> HVFIRTELSFIKNNVPCIRDMFFIYKRELYNICLDDLKGEEDETHIYVQKKVKDSWITLNDLFKETDLTGRPHIFAYVDVEEIIILLCEDEEFSNRKKDMTCHRFYSNDGKEYQNSEITISDYILKDKLLSSYVSLPLKIENREYFLICGVSPYKFK;> HVFIRTELSFIKNNVPCIRDMFFIYKRELYNICLDDLKGEEDETHIYVQKKVKDSWITLNDLFKETDLTGRPHIFAYVDVEEIIILLCEDDEFSNRKKDMTCHRFYSNDGKEYQNSEITISDYILKDKLLSSYVSLPLKIENREYFLICGVSPYKFKDDNK;> DDNKKDDILCMASHDKGETWGTKIVIKYDNYKLGVQYFFLRPYISKNDLSFHFYVGDNINNVKNVNFIECTHEKDLEFVCSNRDFLKDNKVLQDVSTLNDEYIVSYGNDNNFAECYIFFNNENSILIKPEKYGQTTAGCYGGTFVKIDEQRTLFIYSSSQGIYNIHTIYYANYEEF;> KDDILCMASHDKGETWGTKIVIKYDNYKLGVQYFFLRPYISKNDLSFHFYVGDNINNVKNVNFIECTHEKDLEFVCSNRDFLKDNKVLQDVSTLNDEYIVSYGNDNNFAECYIFFNNENSILIKPEKYGNTTAGCYGGTFVKIDEQRTLFIYSSSQGIYNIHTIYYANYE

Sequencing and annotation of the P. falciparum genome has supported the identification of new blood-stage vaccine candidate antigens, among which the P. falciparum Cysteine-Rich Protective Antigen (PfCyRPA) has a number of noteworthy properties. PfCyRPA is part of a multi-protein complex including also the PfRH5-interacting protein PfRipr and the reticulocyte binding-like homologous protein PfRH5, which binds to the erythrocyte receptor basigin. Moreover, PfCyRPA-specific monoclonal antibodies (mAb) inhibit parasite growth both in vitro and in vivo by blocking merozoite invasion. Here, we describe the crystal structure of the promising vaccine candidate PfCyRPA alone and in complex with the antigen-binding fragment (Fab) of the parasite growth inhibitory mAb c12.

In order to crystallize PfCyRPA, we needed to pre-treat the protein with Actinase E. The crystal structure of PfCyRPA, determined to a resolution of 2.5 Å (detailed in Supplementary file 1), confirmed our biophysical analyses. PfCyRPA adopts a six-bladed β-propeller structure that buries the disulfide bonds and the Trp residues. Each blade of the propeller is constructed by a four-stranded anti-parallel β-sheet. The five disulfide bonds in PfCyRPA are located within blades 2–6, stabilizing each individual blade. The first blade has no disulfide bond; it is formed by β-strands from the N- and C-terminal regions of PfCyRPA, potentially enabling conformational changes in PfCyRPA by opening and closing. A domain alignment search (DALI; [Holm and Rosenström, 2010]) for related structures revealed that PfCyRPA adopts a heavily modified sialidase/neuraminidase fold. The closest structural relative is the catalytic domain of Vibrio cholerae sialidase. Two molecules of PfCyRPA are present in the asymmetric unit and have conformational differences in several surface loops, suggesting possible flexibility of these loops in solution. PfCyRPA contains none of the residues necessary for catalysis, nor does it harbor a Ca2+ binding site, providing structural correlates of the absence of sialidase activity in PfCyRPA.>TITARHTQYSHAKTGGFSQTGPTLHNPYKDDPILDRTLRRLLPESEYMRVAADLSKFGDRITSEVEHLGRQAELEQPRLEHQDAWGKRVDKLIVCNEWHKLKQICAEEGVISIGYEDSVDP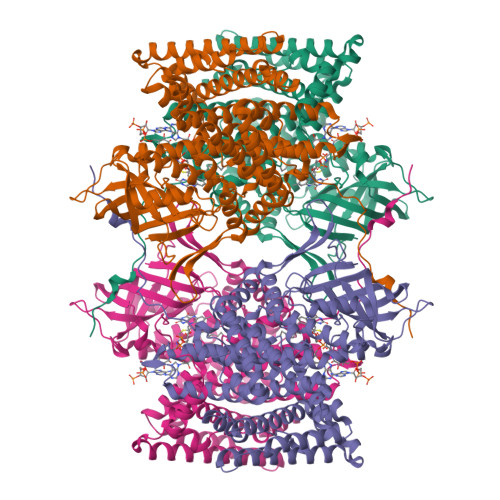FVRRIHQVAKLFLFSPSAGLVSCPMAMTDGAVKTLTSLNLYGKHKLATEAVDRLRSRDPSKAWTSGQWMTEKKGGSDVAGGCDTYAVQIDKDTYRLHGYKWFSSAVDADVALTLARIVDSDGNALEGSRGLSLFLLKIRDESGNLNGIQMVRLKNKLGTKQLPTAELLLDGAIAERIGDQGRGVAGISNMLNITRIHNAVASLGYMRRIISLARDYSTKRVVFGQTQSKWPLHTTTLAKMEVDTRGSMLLLFEAARLLGLSEAGKSSDVEAMMLRLITPVLKLYAGKQAVPMVSEGIECFGGQGYMEDTGLPTLLRDAQVTPIWEGTTNVLSLDVLRVFSGKENILLAFGKRVEQLLGNTKTEDEKLKKSKEAVESALKQLQKLLVKASDSAIQGETRIDSVARHIAFTIARIYSGALLIDHASDSSVANQSDIEVAYRYCCEQPLIDLRWEWFASERVKADREIVFDNFTA[2x]2-[2-[[3-(1~{H}-benzimidazol-2-ylamino)propylamino]methyl]-4,6-bis(chloranyl)indol-1-yl]ethanol 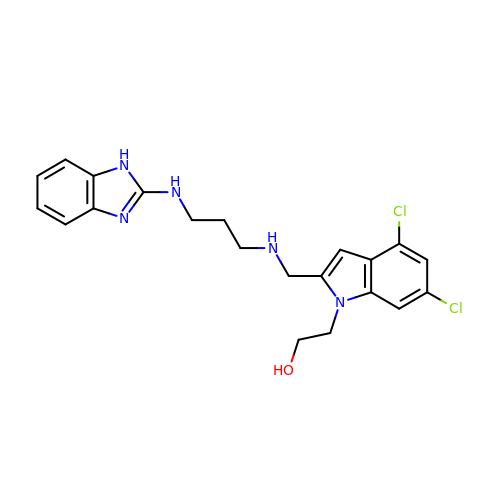| C21 H23 Cl2 N5 O | JCEOIIIPEPYSSD-UHFFFAOYSA-N>HHHHHHMDDSRSVNSVLL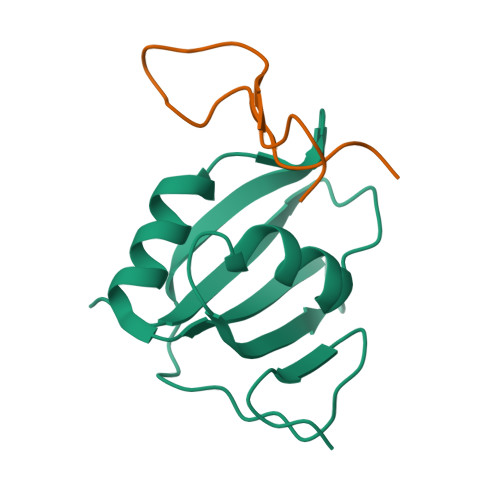FTILNPIYSITTDVLYTICNPCGPVQRIVIFRKNGVQAMVEFDSVQSAQRAKASLNGADIYSGCCTLKIEYAKPTRLNVFKNDQDTWDYTNPN[2x];>[2x]YPPGYPMQAYVDPSNPNAGKVLLPTP> MVQRWLYSTNAKDIAVLYFMLAIFSGMAGTAMSLIIRLELAAPGSQYLHGNSQLFNVLVVGHAVLMIFFLVMPALIGGFGNYLLPLMIGATDTAFPRINNIAFWVLPMGLVCLVTSTLVESGAGTGWTVYPPLSSIQAHSGPSVDLAIFALHLTSISSLLGAINFIVTTLNMRTNGMTMHKLPLFVWSIFITAFLLLLSLPVLSAGITMLLLDRNFNTSFFEVSGGGDPILYEHLFWFFGHPEVYILIIPGFGIISHVVSTYSKKPVFGEISMVYAMASIGLLGFLVWSHHMYIVGLDADTRAYFTSATMIIAIPTGIKIFSWLATIHGGSIRLATPMLYAIAFLFLFTMGGLTGVALANASLDVAFHDTYYVVGHFHYVLSMGAIFSLFAGYYYWSPQILGLNYNEKLAQIQFWLIFIGANVIFFPMHFLGINGMPRRIPDYPDAFAGWNYVASIGSFIATLSLFLFIYILYDQLVNGLNNKVNNKSVIYNKAPDFVESNTIFNLNTVKSSSIEFLLTSPPAVHSFNTPAVQS;> DVPTPYACYFQDSATPNQEGILELHDNIMFYLLVILGLVSWMLYTIVMTYSKNPIAYKYIKHGQTIEVIWTIFPAVILLIIAFPSFILLYLCDEVISPAMTIKAIGYQWYWKYEYSDFINDSGETVEFESYVIPDELLEEGQLRLLDTDTSMVVPVDTHIRFVVTAADVIHDFAIPSLGIKVDATPGRLNQVSALIQREGVFYGACSELCGTGHANMPIKIEAVSLPKFLEWLNEQ;> MTHLERSRHQQHPFHMVMPSPWPIVVSFALLSLALSTALTMHGYIGNMNMVYLALFVLLTSSILWFRDIVAEATYLGDHTMAVRKGINLGFLMFVLSEVLI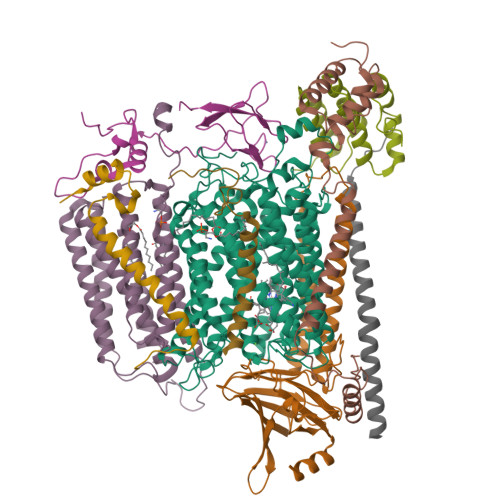FAGLFWAYFHSAMSPDVTLGACWPPVGIEAVQPTELPLLNTIILLSSGATVTYSHHALIAGNRNKALSGLLITFWLIVIFVTCQYIEYTNAAFTISDGVYGSVFYAGTGLHFLHMVMLAAMLGVNYWRMRNYHLTAGHHVGYETTIIYTHVLDVIWLFLYVVFYWWGV;> PVVKTAQNLAEVNGPETLIGPGAKEGTVPTDLDQETGLARLELLGKLEGIDVFDTKPLDSSRKGTMKDPIIIESYDDYRYVGCTGSPAGSHTIMWLKPTVNEVARCWECGSVYKLNPVGVP;> AQTHALSNAAVMDLQSRWENMPSTEQQDIVSKLSERQKLPWAQLTEPEKQAVWYISYGEWGPRRPVLNKGDSSFIAKGVAAGLLFSVGLFAVVRMAGGQDAKTMNKEWQLKSDEYLKSKNANPWGGYSQVQSK;> DEETFEEFTARYEKEFDEAYDLFEVQRVLNNCFSYDLVPAPAVIEKALRAARRVNDLPTAIRVFEALKYKVENEDQYKAYLDELKDVRQELGVPLKEELFPSSS;> ANKVIQLQKIFQSSTKPLWWRHPRSALYLYPFYAIFAVAVVTPLLYIPNAIRGIKAKKA;> VHFKDGVYENIPFKVKGRKTPYALSHFGFFAIGFAVPFVACYVQLKK;> TIAPITGTIKRRVIMDIVLGFSLGGVMASYWWWGFHMDKINKREKFYAELAERKK>GAMGSEQRASLDSEESESPPQENSCLDPPDRDPNCKPPPVKPHIFTTRSRTRLFGKGDSEEASPLDCPYEEGGLASCPIITVSSVLTIQRPGDGPASVRPSSQDSVSAGEKPPRLYDRRSIFDAVAQSNCQELESLLPFLQRSKKRLTDSEFKDPETGKTCLLKAMLNLHNGQNDTIALLLDVARKTDSLKQFVNASYTDSYYKGQTALHIAIERRNMTLVTLLVENGADVQAAANGDFFKKTKGRPGFYFGELPLSLAACTNQLAIVKFLLQNSWQPADISARDSVGNTVLHALVEVADNTVDNTKFVTSMYNEILILGAKLHPTLKLEEITNRKGLTPLALAASSGKIGVLAYILQREIHEPECRHLSRKFTEWAYGPVHSSLYDLSCIDTCEKNSVLEVIAYSSSETPNRHDMLLVEPLNRLLQDKWDRFVKRIFYFNFFVYCLYMIIFTAAAYYRPVEGLPPYKLKNTVGDYFRVTGEILSVSGGVYFFFRGIQYFLQRRPSLKSLFVDSYSEILFFVQSLFMLVSVVLYFSQRKEYVASMVFSLAMGWTNMLYYTRGFQQMGIYAVMIEKMILRDLCRFMFVYLVFLFGFSTAVVTLIEDGKNNSLPMESTPHKCRGSACKPGNSYNSLYSTCLELFKFTIGMGDLEF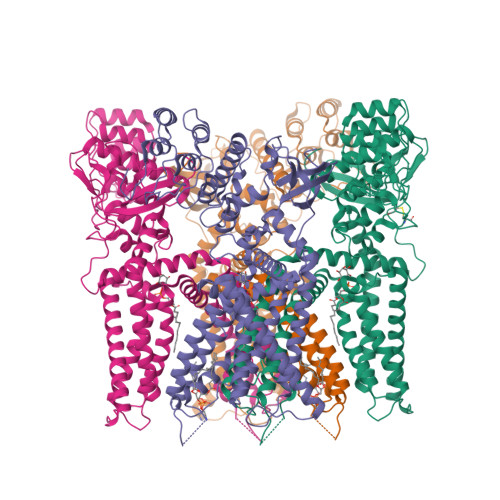TENYDFKAVFIILLLAYVILTYILLLNMLIALMGETVNKIAQESKNIWKLQRAITILDTEKSFLKCMRKAFRSGKLLQVGFTPDGKDDYRWCFRVDEVNWTTWNTNVGIINEDPGNCEGVKRTLSFSLRSGRVSGRNWKNFALVPLLRDASTRDRHATQQEEVQLKHYTGSLKPEDAEVFKDSMVPGEK[4x]> MAQALPWLLLWMGAG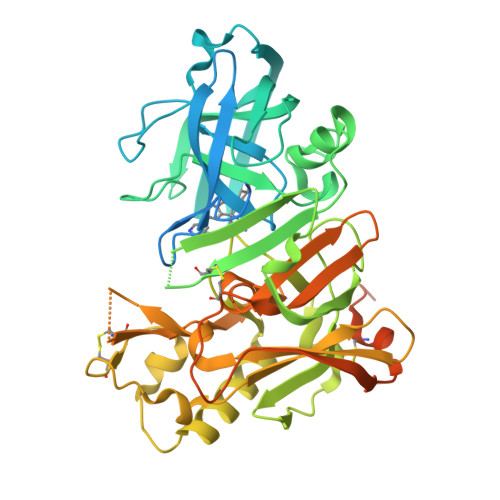VLPAHGTQHGIRLPLRSGLGGAPLGLRLPRETDEEPEEPGRRGSFVEMVDNLRGKSGQGYYVEMTVGSPPQTLNILVDTGSSNFAVGAAPHPFLHRYYQRQLSSTYRDLRKGVYVPYTQGKWEGELGTDLVSIPHGPNVTVRANIAAITESDKFFINGSNWEGILGLAYAEIARPDDSLEPFFDSLVKQTHVPNLFSLQLCGAGFPLNQSEVLASVGGSMIIGGIDHSLYTGSLWYTPIRREWYYEVIIVRVEINGQDLKMDCKEYNYDKSIVDSGTTNLRLPKKVFEAAVKSIKAASSTEKFPDGFWLGEQLVCWQAGTTPWNIFPVISLYLMGEVTNQSFRITILPQQYLRPVEDVATSQDDCYKFAISQSSTGTVMGAVIMEGFYVVFDRARKRIGFAVSACHVHDEFRTAAVEGPFVTLDMEDCGYNIPQTDESTLMTIAYVMAAICALFMLPLCLMVCQWRCLRCLRQQHDDFADDISLLK> MLRRTSWRAVGYTPVNPDTSPMLAYSQYHWHYNLPQGMERPHGVNRTMTAPYQSAHSLVNKYRGVWIELDMHPAFRVALEPQLRKLPQGRTIPKTSVDEVISDYINTAHLIQDEMTRDLWLAKVLQHCAFQRSNEGMALWEKYCHSRFIADGATATPPLPLVKAILFYCSKIDYQGWSSIFQKCLKNDWNYTPLFDTAQWNFLLKSVGRMGDEKGVRLILEEMLDVQADLDRVEARSIVIALNAVTDNDIYEYIKK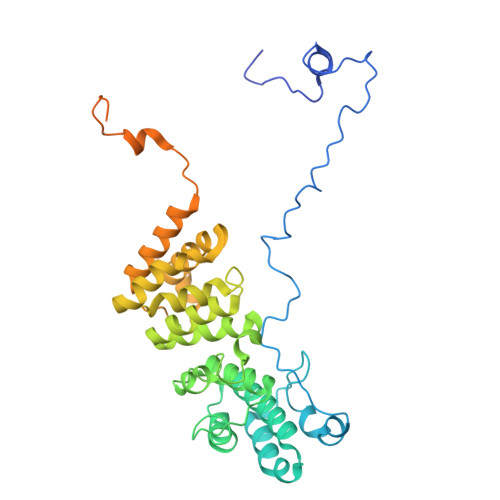YLFNFGERKVKFLRIIYSDLRGHGAGKLRIPLKENDKMFYHVCWHSSIRAPRQFSPRQLYFDYTPSTLGASVHNPNAKIDDIVKDKIEKWKTEGLLPEDYVHEDRVYDRGTAFKNVARQEKWKKMPRIVKSKKMGYTGDP> MGSDSIDTPNYDVQKHINKLCGMLLITEDANHKFTGLIGMLYAMSRLGREDTIKILRDAGYHVKANGVDVTTHRQDINGKEMKFEVLTLASLTTEIQINIEIESRKSYKKMLKEMGEVAPEYRHDSPDCGMIILCIAALVITKLAAGDRSGLTAVIRRANNVLKNEMKRYKGLLPKDIANSFYEVFEKHPHF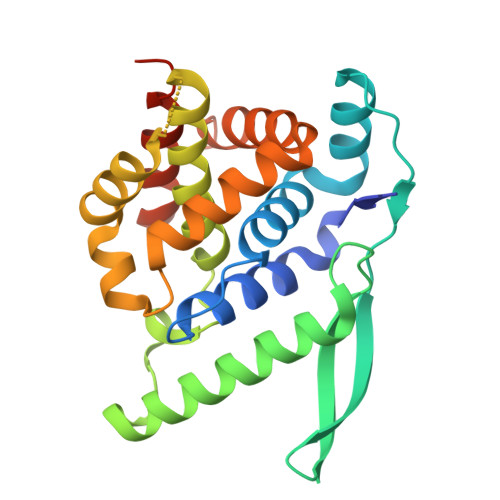IDVFVHFGIAQSSTRGGSRVEGIFAGLFMNAYGLEHHHHHH Of particular interest are the Esx complexes which are dimers of two subunits (ESAT-6, early secreted antigen of 6 kDa; and CFP-10, culture filtrate protein of 10 kDa) and which are secreted across the cytoplasmic membrane by Type VII secretion (T7S) systems. Mycobacterial ESX secretion systems have been shown to be involved in a variety of physiological processes including conjugation in a non-pathogenic mycobacterium, iron and/or zinc acquisition by both pathogenic and non-pathogenic mycobacterial species, and virulence of pathogenic mycobacteria. The overall architecture of the complexes is similar to known Esx structures in that each heterodimer forms a four helix bundle with the CFP-10 and ESAT-6 subunit homologs each contributing an α-helical hairpin to the complex. The subunit interfaces in the four-helix bundles of the Esx complexes are similar to those of the previously determined Esx complex structures in that the intermolecular interface between the CFP-10 and ESAT-6 subunits is largely hydrophobic.

Using this expression approach we expressed and purified six Esx complexes and determined the crystal structures of M. abscessus EsxEF (EsxEFma), encoded by the MAB_3112 and MAB_3113 genes, M. smegmatis EsxGH (EsxGHms), encoded by the MSMEG_0620 and MSMEG_0621 genes, and M. tuberculosis EsxOP (EsxOPmt), encoded by the Rv2346c and Rv2347c genes, at resolutions of 1.96 Å, 2.70 Å, and 2.55 Å, respectively. The structures of these complexes were determined by single wavelength anomalous diffraction (EsxEFma and EsxGHms) and multiple wavelength anomalous diffraction (EsxOPmt) at resolutions of 3.0 Å, 2.70 Å, and 2.55 Å, respectively. The asymmetric units for the EsxEFma crystal forms have a single complex in the asymmetric unit for the SeMet-labeled protein and six complexes in the asymmetric unit of the native protein crystal form while the EsxGHms and EsxOPmt (both crystal forms) contain two heterodimeric complexes. The WXG-containing loops are well ordered in the EsxGHms complexes and in most of the EsxEFma complexes but the majority of the connecting loops are disordered in the EsxOPmt subunit structures. Additional regions of disorder are found at the N- and C-termini of the complexes with the EsxFma and EsxOmt subunits having a substantial number of disordered residues at their C-termini. The average amount of buried surface area in the subunit interfaces varies considerably [EsxEFma, ∼1605 Å2; EsxGHms, ∼1555 Å2; EsxOPmt (form I), ∼1025 Å2; and EsxOPmt (form II), ∼1175 Å2] and the percentage of the surface of each subunit buried in the complex interface is also highly variable, from 13.5–33%, and is related to the degree to which the termini of the subunits are ordered and to the conformations that they adopt.

>[2x]MTINYQFGDVDAHGAMIRAQAGLLEAEHQAIVRDVLAAGDFWGGAGSVACQEFITQLGRNFQVIYEQANAHGQKVQAAGNNMAQTDSAVGSSWATHHHHHH;>[2x]SMATRFMTDPHAMRDMAGRFEVHAQTVEDEARRMWASAQNISGAGWSGMAEATSLDTMAQMNQAFRNIVNMLHGVRDGLVRDANNYEQQEQASQQILSS> MHHHHHHIRSFSCADTEALFTTGKTRRGSDIKSVAERKLAMLDAATELRDLRSPPGNRLESLSGNRADQHSIRVNDQWRLCFTWTEH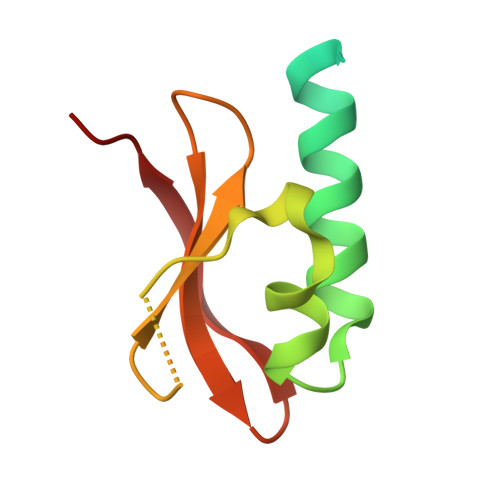GPVNVEIVDYH>GKTEVKQQSESELKHYYNKPVLERKNVTGYKYTEKGKDYIDVIVD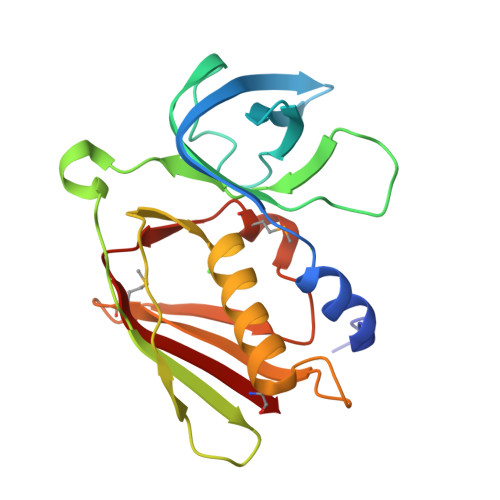NQYSQISLVGSDKDKFKDGDNSNIDVFILREGDSRQATNYSIGGVTKTNSQPFIDYIHTPILEIKKGKEEPQSSLYQIYKEDISLKELDYRLRERAIKQHGLYSNGLKQGQITITMKDGKSHTIDLSQKLEKERMGDSIDGRQIQKILVEMK[2x]> NNAFCAGFGLSCKWECWCTAHGTGNELRYATAAGCGDHLSKSYYDARAGHCLFSDDLRNQ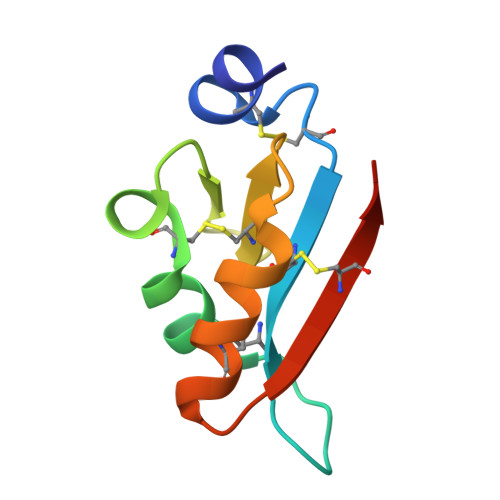FYSHCSSLNNNMSCRSLSKR> AALRERAGPVTWVMMIACVVVFIAMQILGDQEVMLWLAWPFDPTLKFEFWRYFTHALMHFSLMHILFNLLWWWYLGGAVEKRLGSGKLIVITLISALLSGYVQQKFSGPWFGGLSGVVYALMGYVWLRGERDPQSGIYLQRGLIIFALIWIVAGWFDLF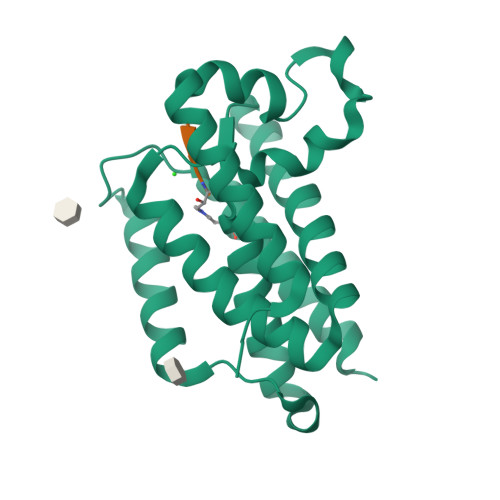GMSMANGAHIAGLAVGLAMAFVDSLNARKRKASLERENLYF>RLSLEHAIGTVCHPSLMNVDAAVGGLNRDPVEAANPYGAYVAAPAGPAADMQQLFLNAWGQRLAHGRVRWVAEGQMTPEQFMQPDNANLALELHPAFDFFVGVADVELPGGDVPPAGPGEIQATWRVVNGNLPLALCPAAFRDARGLELGVGRHAMAPATIAAVRGAFDDRNYPAVFYLLQAAIHGSEHVFCALARLVVQCITSYWNNTRCAAFVNDYSLVSYVVTYLGGDLPEECMAVYRDLVAHVEALAQLVDDFTLTGPELGGQAQAELNHLMRDPALLPPLVWDCDALMRRAALDRHRDCRVSAGGHDPVYAAACNVATAD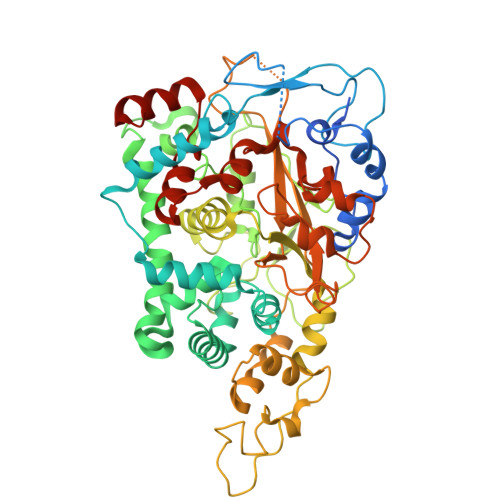FNRNDGQLLHNTQARAADAADDRPHRGADWTVHHKIYYYVMVPAFSRGRCCTAGVRFDRVYATLQNMVVPEIAPGEECPSDPVTDPAHPLHPANLVANTVNAMFHNGRVVVDGPAMLTLQVLAHNMAERTTALLCSAAPDAGANTASTTNMRIFDGALHAGILLMAPQHLDHTIQNGDYFYPLPVHALFAGADHVANAPNFPPALRDLSRQVPLVPPALGANYFSSIRQPVVQHVRESAAGENALTYALMAGYFKISPVALHHQLKTGLHPGFGFTVVR[2x]> VTSYTLSD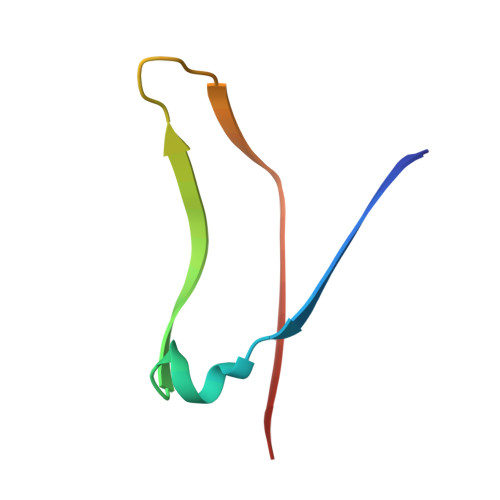VVSLKDVVPEWVRIGFSATTGAEYAAHEVLSWSFHSELS> RLMTRIALDPFVRDLDGESAALRAAGPLAEVELPGGVHVYAVTRHAEARALLTDSRVVKDIDVWNAWRRGEIPMDWPLIGLANPGRSMLTVDGADHRRLRTLVAQALTVKRVERLRAGIEALTNASLEKLAALPAGEPVDLKAEFAYPLPMNVISELMGVDAADHPRLKELFEKFFSTQTPPEEVPQMMADLGALFTKIVDAKRTNPGDDLTSALIAASENGDHLTDEEIVNTLQLIIAAGHETTI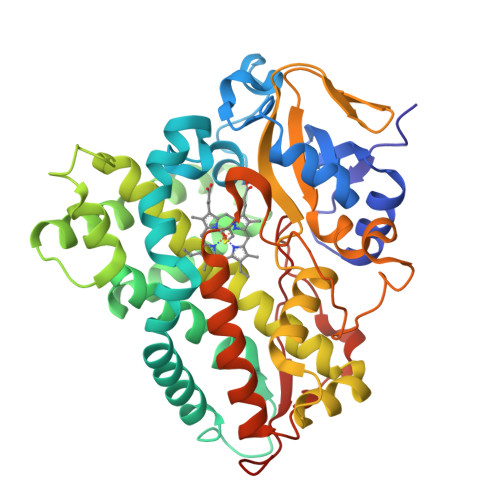SLIVNVVEALQTHPEQRKKVLNGEIGWDGVIEETLRWNTPTSHVLIRFATEDIEVGDKILPKGEGLIISFGALGRDEEQYGPTAGEFDATRTPNRHIAFGHGPHVCPGAALSRLEAGIALPALYERFPELDLAVPASDLRNKPIVTQNDLHELPVKLGCPFGGDA>[6x]AVSVALGQTVRITCQGDSLRSYSASWYQQKPGQAPVLVIFRNTASLTITGAQAEDEADYYCNSRDSSANHQVFGGGTKLTV

We here present the cryo-EM structures of two amyloid fibrils (A and B) that were extracted from the explanted heart of a patient (FOR005) with systemic AL amyloidosis. The tissue-deposited fibril protein consists of residues Ser2–Ser116 of the λ3 precursor LC, which correspond to the VL domain and a few residues (Gly109–Ser116) of the LC constant (CL) domain. 2D projections of the models correspond well to the 2D class averages of the original segments. Both models depict polar fibrils with C1 helical symmetry, consisting of only one protofilament and a single stack of fibril proteins. Using cryo-EM, we obtained two different fibril structures, termed here A and B. The two structures coexist at different z-axial positions within the same fibril, which implies the presence of structural breaks in these patient-derived amyloid fibrils.

The two fibril structures arise from similar but slightly different protein conformations. The fibril proteins are essentially indistinguishable at residues Ala9–Arg49 and Leu72–Val107. The main difference between the two structures lies in the segment Arg60–Ser71. In fibril B, residues Asn68–Ser71 are in a relatively extended conformation and the region of structural disorder occurs between residues Lys50–Gly67. The corresponding reconstructions were refined to spatial resolutions of 3.2 Å for fibril structure A and 3.4 Å for B, based on the 0.143 Fourier shell correlation (FSC) criterion. We interpreted the two reconstructions with molecular models and obtained model resolutions of 3.1 Å for reconstruction A and 3.2 Å for B. The fibril backbones show axial height changes of 7.5 Å (fibril A) and 7.0 Å (fibril B), which lead to polar fibril topologies and sterically interlock the fibril layers. Surprisingly, however, we found that most fibrils in our sample showed a mixture of A and B segments. Moreover, the segments are not randomly distributed across the fibrils, but mostly separated into distinct regions along the fibril axis, in which all segments correspond to either structure A or B. The other scenario is that breaks emerge after fibril assembly, for example, because initially disordered segments adopt different stable conformations, which then proliferate along the fibril axis. Support for the latter mechanism is provided by the fact that the type A and B fibril proteins are mostly identical, and that the differences are confined to a small segment that lies in the vicinity of an unstructured region.>SDKIIHLTDDSFDTDVLKADGAILVDFWAEWCGPCKMIAPILDEIADDYQGKLTVAKLNIDQNPGTAPKY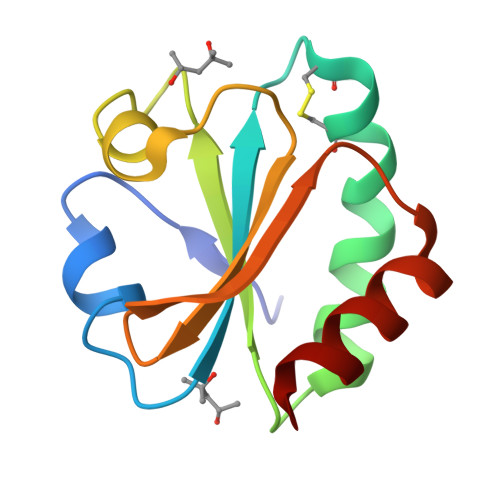GIRGIPTLLLFKNGEVAATKVGALSKGQLKEFLDANLA[2x]> MKVNNTIVVSIGQAGNQIAASFWKTVCLEHGIDPLTGQTAPGVAPRGNWSSFFSKLGESSSGSYVPRAIMVDLEPSVIDNVKATSGSLFNPANLISRTEGAGGNFAVGYLGAGREVLPEVMSRLDYEIDKCDNVGGIIVLHAIGGGTGSGFGALLIESLKEKYGEIPVLSCAVLPSPQVSSVVTEPYNTVFALNTLRRSADACLIFDNEALFDLAHRKWNIESPTVDDLNLLITEALAGITASMRFSGFLTVEISLRELLTNLVPQPSLHFLMCAFAPLTPPDRSKFE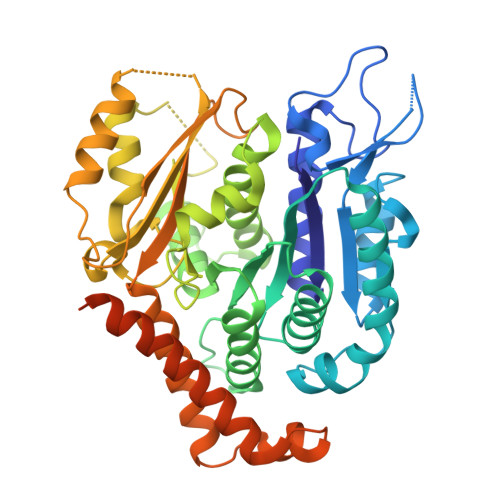ELGIEEMIKSLFDNGSVFAACSPMEGRFLSTAVLYRGIMEDKPLADAALAAMREKLPLTYWIPTAFKIGYVEQPGISHRKSMVLLANNTEIARVLDRICHNFDKLWQRKAFANWYLNEGMSEEQINVLRASAQELVQSYQVAEESGAKAKVQDSAGDTGMRAAAAGVSDDARGSMSLRDLVDRRR>MTKQYKNYVNGEWKLSENEIKIYEPASGAELGSVPAMSTEEVDYVYASAKKAQPAWRALSYIERAAYLHKVADILMRDKEKIGAILSKEVAKGYKSAVSEVVRTAEIINYAAEEGLRMEGEVLEGGSFEAASKKKIAVVRREPVGLVLAISPFNYPVNLAGSKIAPALIAGNVIAFKPPTQGSISGLLLAEAFAEAGLPAGVFNTITGRGSEIGDYIVEHQAVNFINFTGSTGIGERIGKMAGMRPIMLELGGKDSAIVLEDADLELTAKNIIAGAFGYSGQRCTAVKRVLVMESVADELVEKIREKVLALTIGNPEDDADITPLIDTKSADYVEGLINDANDKGATALTEIKREGNLICPILFDKVTTDMRLAWEEPFGPVLPIIRVTSVEEAIEISNKSEYGLQASI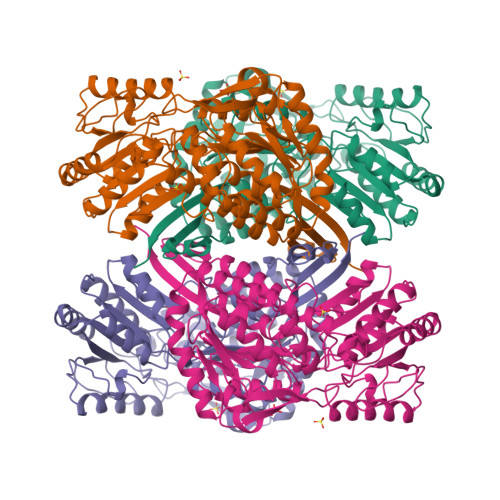FTNDFPRAFGIAEQLEVGTVHINNKTQRGTDNFPFLGAKKSGAGIQGVKYSIEAMTTVKSVVFDIK[4x]>[3x]MTIHSCLARRAVSVAASGARAFASGLGARAVAVGALQSARLLHTSSLRAAGAKISPSEMSRLLEERIAGWKTQTSTEEVGRVVSVGDGIARLFGLEGVQAGELVEFQNGMTGMALNLETDNVGVVIFGDDRSVLEGDSVKRTGRIVDVPIGPGLLGRVVDALGNPIDGKGPIPAKERRRVELKAPGIIPRKSVHEPMMTGLKCVDALVPVGRGQRELIIGDRQTGKTAVAVDAIINQKEINDSTDDESKKLYCIYVAVGQKRSTVAQIVKALEQRDAMKYTTVVAATASEAAPLQFLAPYSGCAMGEWFRDSGRHCVIIYDDLSKQATAYRQMSLLLRRPPGREAYPGDVFYLHSRLLERAAKMGDKSGGGSLTALPVIETQAGDVSAYIPTNVISITDGQIFLETELFYKGIRPAINVGLSVSRVGSAAQVKAMKQVAGTMKLELAQYREVAAFAQFGSDLDASTRQLLTRGTALTELLKQRQYSPMKNSVQVCVLYCGVKGYLDPLDPKEISRFESLFIDYINANHQDILKTIETEKELSEKTEAKLRAAVDEFVAMNEFKKK;>MASPALQTCWRNLARLSGAQVRPSHFGAFSLGSRMSPFSSLLGARASPIATGRAGLRFLSSAAPNPGKKPASAAPPAGTNHGRITQVIGAVVDVHFDEQLPPILNSLEVQGHTNRLVLEVAQHLGENTVRTIAMDATEGLVRGQKVVDTGAPIQVPVGVETLGRIMNVIGEPVDECGPVPAKKTYSIHRAAPLFADQSTEPGLLQTGIKVVDLLAPYAKGGKIGLFGGAGVGKTVLIMELINNVANKHGGFSVFAGVGERTREGNDLYHEMMTTGVIKRKKLEDGKFDFTGSKAALVYGQMNEPPGARARVALTALSVAEYFRDEQGQDVLLFIDNIYRFTQAGSEVSALLGRIPSAVGYQPTLATDL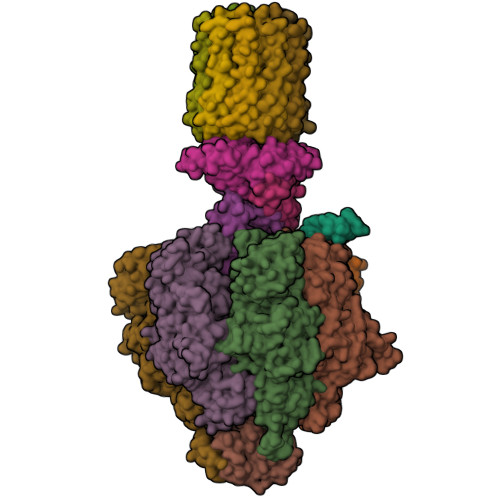GQLQERITTTKKGSITSVQAVYVPADDLTDPAPATTFAHLDATTVLSRQIAELGIYPAVDPLDSTSRMLAPEIVGQEHYDTARATQKLLQDYKSLQDIIAILGMDELSEEDKLVVSRARKIQRFLSQPFTVAEVFTGKPGRFVELPETIKSAQTILRGECDDLPEMAFYMCGGLEEVRSKAVKMAQEAASGK[3x];> MALPLLASRRLFSSFVFRGQPSTLSSNLSLVRIRGLHGGSLSPPSATLPRAVQLFSSRIAFSTAAAEDSGASQTLEGRYASALFRVAKKKNQLEKVYGDLESVRNALKDSSEFRLFVDSPAVSVQQKLDVLRQLVNRYKFDPLTGNLLTTLVENKRLPMLARVADAFDAMYRKEKGEVKCLVTSAKPLSAQQQKEIVAALQNRAGTQARLIIDYAVSPQIMGGLVVRLGEQVLDFSVATRLDRLQSQLLAPL;>[10x]MFFSRLSLSALKAAPAREALPGLLSRQSFSSAGFSQFSSQKFFFSPSRNFSQSPLFQKHTPVHCNQRIASALVPTQQPAMTRQNPYAMQVGARYDAGVASLSAAIALMSVGGVAQGIGSLFAALVSGTARNPSIKEDLFTYTLIGMGFLEFLGIICVLMSAVLLYS;> MFARAFSRFASLAAPAPQRGWNAFVLPSRHFATAAGGANPFKNQLLLTLSSPSEAIYVRTPVRSVTVPGSEGAMTMTNGHSQTVARLKAGEIIVRKGETGDEVERFFLSDGFVLFKSPEDDSGCCTAEVLGVEVVPVSMLDKESAATALQELLQQGAGATDEWTKARTLLGQELLSSVIRAAP;> MWRSSGVSFTRYASEMAALLRQCLKEPYRTQAMQRNQIHLKETVYQQGQVLTRETFNDIKKAFEAAAKHAGEK;> MAGLASLSSVGALRGMRLVPAAHLLPLHSAFGQQTRNFGAGDLKIVAARMKSVKSIQKITKAMKMVAASKLRMDQRRLENGLPFATPVQKLVQRIPVDPKEKGTLAVLALSSDKGLCGGVNSFVAKQARIVIKENEMAGNAVQVYGVGDKIRSALQRTFGDRFKRIMTEVTRFPWNFGQACIIADRLMQDNPARLMVIYNHFKSAVAYDTLTLNVLTPTQAAQSAKEQLNTFEFEPEKTDVWKDLQDFYYACTVFGCMLDNIASEQSARMSAMDNASTNAGEMISSLTLRYNRARQAKITTELVEIISGANALE;> MSSPCCVAIRRVARTTLESGRRQVDSKSTDVSPFFTGTQQMSLPSAGMVTKIRNFSSVKFMDQKRSGEETVYFKKEDEALLRNLLANHPEYDPKYSVDHMNAEVGSIARDITLACQKHGMKDPSAAFMKDLISIFGAHGYAKNSK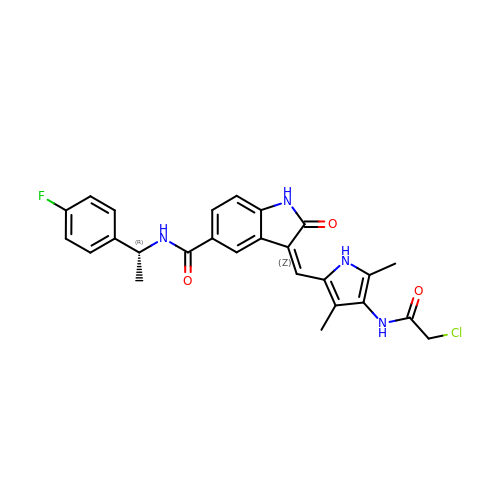(3Z)-3-{[4-(2-chloroacetamido)-3,5-dimethyl-1H-pyrrol-2-yl]methylidene}-N-[(1R)-1-(4-fluorophenyl)ethyl]-2-oxo-2,3-dihydro-1H-indole-5-carboxamide | C26 H24 Cl F N4 O3 | IDWBLFLYQVHAFH-LPKQHDGYSA-N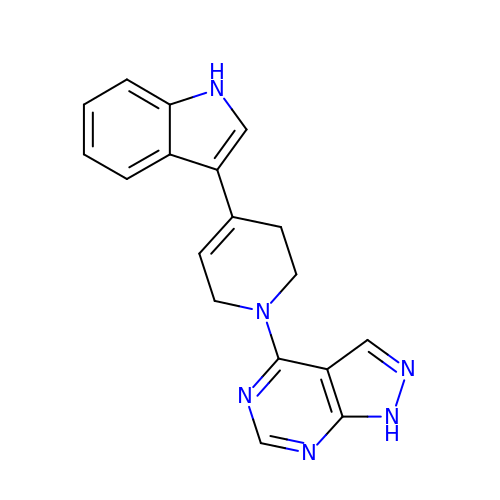4-[4-(1H-indol-3-yl)-3,6-dihydropyridin-1(2H)-yl]-1H-pyrazolo[3,4-d]pyrimidine | C18 H16 N6 | QOXYIHCPHZOWJH-UHFFFAOYSA-N>[2x]MTKYALVGDVGGTNARLALCDIASGEISQAKTYSGLDYPSLEAVIRVYLEEHKVEVKDGCIAIACPITGDWVAMTNH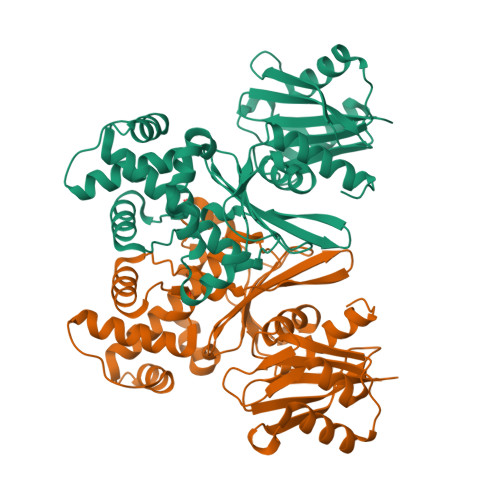TWAFSIAEMKKNLGFSHLEIINDFTAVSMAIPMLKKEHLIQFGGAEPVEGKPIAVYGAGTGLGVAHLVHVDKRWVSLPGEGGHVDFAPNSEEEAIILEILRAEIGHVSAERVLSGPGLVNLYRAIVKADNRLPENLKPKDITERALADSCTDCRRALSLFCVIMGRFGGNLALNLGTFGGVFIAGGIVPRFLEFFKASGFRAAFEDKGRFKEYVHDIPVYLIVHDNPGLLGSGAHLRQTLGHILHHHHHH The RoboDiff forms the core of the services offered on the ESRF beamline MASSIF-1 and, thus far, has been used to mount, characterize and collect diffraction data from over 20 000 samples since September 2014. In all three cases diffraction images were indexed and integrated using XDS and reduced using AIMLESS.

ARP/wARP was then run for automatic model building. Both models were completed manually using Coot interspersed with refinement with REFMAC5.

> MASDKFPVAENPSSSFKYESAVQYRPAPDSYLNPCPQAGRIVKETYTGINGTKSLNVYLPYGYDPNKKYNIFYLMHGGGENENTIFSNDVKLQNILDHAIMNGELEPLIVVTPTFNGGNCTAQNFYQEFRQNVIPFVESKYSTYAESTTPQGIAASRMHRGFGGFSMGGLTTWYVMVNCLDYVAYFMPLSGDYWYGNSPQDKANSIAEAINRSGLSKREYFVFAATGSEDIAYANMNPQIEAMKALPHFDYTSDFSKGNFYFLVAPGATHWWGYVRHYIYDALPYFFHELEHHHHHH HVEM is a TNF (tumor necrosis factor) receptor contributing to a broad range of immune functions involving diverse cell types. It interacts with a TNF ligand, LIGHT, and immunoglobulin (Ig) superfamily members BTLA and CD160. HVEM engages in bidirectional signaling, serving not only as a receptor but also as a ligand for IgSF receptor signaling. To dissect the molecular basis for multiple functions, we determined crystal structures that reveal the distinct HVEM surfaces that engage LIGHT or BTLA/CD160, including the human HVEM–LIGHT–CD160 ternary complex, with HVEM interacting simultaneously with both binding partners.

Mixing equal molar equivalents of hLIGHT and hHVEM monomers resulted in a single species with an apparent molecular weight of ∼100 kD, consistent with the formation of a 3:3 stoichiometric hHVEM–hLIGHT assembly in solution. The asymmetric unit of the hHVEM–hLIGHT crystals contains six independent chains of hLIGHT and six independent chains of hHVEM, which form two classical 3:3 TNF–TNFR hexameric assemblies with threefold symmetry; a single 3:3 TNF–TNFR hexameric assembly is consistent with SEC analysis. The hHVEM ectodomain is composed of four cysteine-rich domains (CRDs), while hLIGHT forms a compact homotrimeric structure. In the hexameric assembly, CRD1, CRD2, and CRD3 of hHVEM engage hLIGHT via surfaces contributed by two adjacent hLIGHT protomers. The two independent hHVEM–hLIGHT hexameric complexes exhibit similar overall structures with a root mean square deviation of 1.8 Å for 742 aligned Cα atoms. The hHVEM–hLIGHT recognition interfaces are highly similar within and between the two complexes, and the following discussion is based on the hLIGHT G and H chains and hHVEM J chain. The structure of the hHVEM–hLIGHT complex shows that HVEM CRD1 and CRD2 domains interact with the DE, AA′ and GH loops of LIGHT, while HVEM CRD3 interacts with LIGHT CD and EF loops. The interaction between the hHVEM CRD2 and hLIGHT DE loop appears to be important for hHVEM–hLIGHT recognition, as it contributes multiple potential polar contacts. The main-chain amide group of hHVEM A85 (position numbered with initiation codon = 1) forms a hydrogen bond with the side-chain hydroxyl group of hLIGHT Y173, consistent with the behavior of the Y173F mutation in hLIGHT, which significantly diminishes the binding of hLIGHT with hHVEM. hHVEM N88 does not directly contact hLIGHT Y173 but is relatively close, and the hHVEM N88A mutation attenuated binding to hLIGHT. The hHVEM M98 backbone amide group contacts the backbone oxygen of hLIGHT R228, and the side-chain carboxyl group of hHVEM D100 forms two polar contacts with the side-chain guanidinium group of hLIGHT R226.

>[6x]HHHHHHGLIQERRSHEVNPAAHLTGANSSLTGSGGPLLWETQLGLAFLRGLSYHDGALVVTKAGYYYIYSKVQLGGVGCPLGLASTITHGLYKRTPRYPEELELLVSQQSPCGRATSSSRVWWDSSFLGGVVHLEAGEEVVVRVLDERLVRLRDGTRSYFGAFMV;>[6x]RSLPSCKEDEYPVGSECCPKCSPGYRVKEACGELTGTVCEPCPPGTYIAHLNGLSKCLQCQMCDPAMGLRASRNCSRTENAVCGCSPGHFCIVQDGDHCAACRAYATSSPGQRVQKGGTESQDTLCTGHHHHHH> TQKSLSKEEIERYSRQMIVPGMGKEGQLRLMNAKVLIIGAGGLGCPAAQYLAGAGVGTIGIVDGDSVETSNLHRQVAHATKRVGMLKVDSLITHLIEINPLPVYVPYRFDLTPQNAAQIIKPWDVILDCTDNPATRYLISDVCVLLGKPLVSAASVQKSGQLIVLNCPPTPQGVVNKKAAPCYRCCFKKPPPPSAQTSKGE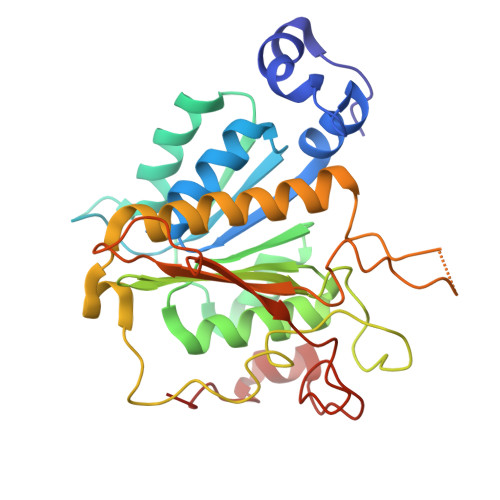AGIMGPVVGMMGVAQAGEAIKILVSQLHMPPKEGEEVSPEKNLVQPTLLIYTYDLNSAIGPYSFRALKMGGRKKDCFACGENSTLTLDGIKSGNPNYVQQ>[2x]MDYKDDDDKMQPDMSLNVIKMKSSDFLESAELDSGGFGKVSLAFHRTQGLMIMKTVYKGPNCIEHNEALLEEAKMMNRLRHSRVVKLLGVIIEEGKYSLVMEYMEKGNLMHVLKAEMSTPLSVKGRIILEIIEGMAYLHGKGVIHKDLKPENILVDNDFHIKIADLGLA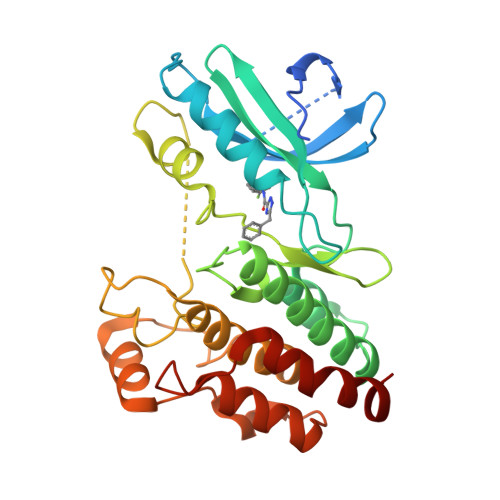SFKMWSKLNNEEHNELREVDGTAKKNGGTLYYMAPEHLNDVNAKPTEKSDVYSFAVVLWAIFANKEPYENAIAEQQLIMAIKSGNRPDVDDITEYCPREIISLMKLCWEANPEARPTFPGIEEKFRPFYLSQLE> P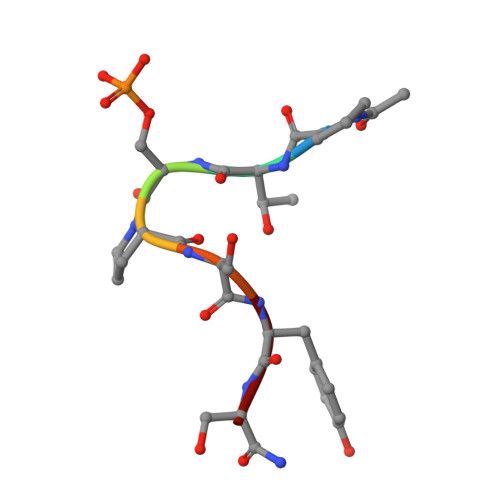TSPSYS>[4x]MTVVPENFVPGLDGVVAFTTEIAEPDKDGGALRYRGVDIEDLVSQRVTFGDVWALLVDGNFG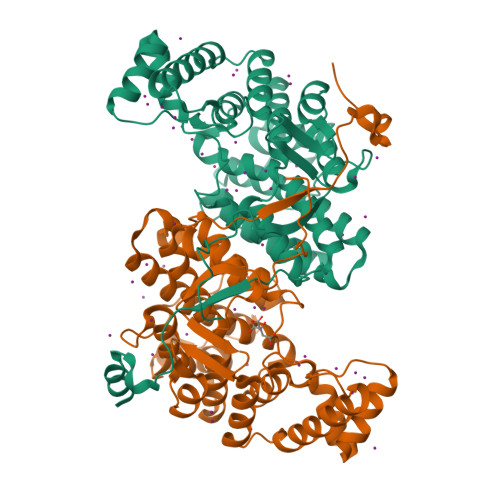SGLPPAEPFPLPIHSGDVRVDVQAGLAMLAPIWGYAPLLDIDDATARQQLARASVMALSYVAQSARGIYQPAVPQRIIDECSTVTARFMTRWQGEPDPRHIEAIDAYWVSAAEHGMNASTFTARVIASTGADVAAALSGAIGAMSGPLHGGAPARVLPMLDEVERAGDARSVVKGILDRGEKLMGFGHRVYRAEDPRARVLRAAAERLGAPRYEVAVAVEQAALSELRERRPDRAIETNVEFWAAVVLDFARVPANMMPAMFTCGRTAGWCAHILEQKRLGKLVRPSAIYVGPGPRSPESVDGWERVLTTAGHHHHHH>[2x]MGIGIYSPGIWRIPHLEKFLAQPCQKLSLLRPVPQEVNAIAVWGHRPSAAKPVAIAKAAGKPVI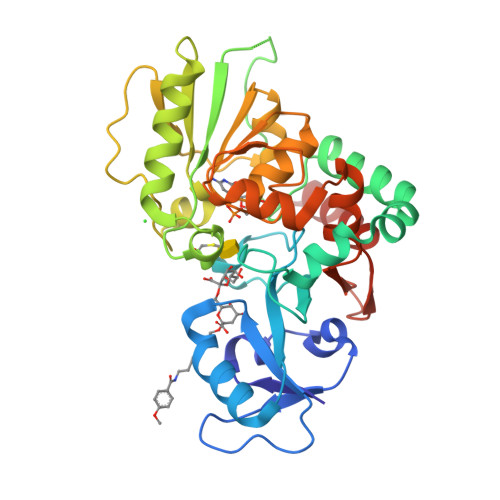RLEDGFVRSLDLGVNGEPPLSLVVDDCGIYYDASKPSALEKLVQDKAGNTALISQAREAMHTIVTGDMSKYNLAPAFVADESERTNIVLVVDQTFNCMSVTYGNAGPHEFAAMLEAAMAENPQAEIWVKVHPDVLEGKKTGYFADLRATQRVRLIAENVSPQSLLRHVSRVYVVTSQYGFEALLAGKPVTCFGQPWYASWGLTDDRHPQSALLSARRGSATLEELFAAAYLRYCRYIDPQTGEVSDLFTVLQWLQLQRRHHHHHH> SSLDDKPQFPGASAEFIDKLEFIQPNVISGIPIYRVMDRQGQIINPSEDPHLPKEKVLKLYKSMTLLNTMDRILYESQRQGRISFYMTNYGEEGTHVGSAAALDNTDLVFGQYREAGVLMYRDYPLELFMAQCYGNISDLGKGRQMPVHYGCKERHFVTISSPLATQIPQAVGAAYAAKRANANRVVICYFGEGAASEGDAHAGFNFAATLECPIIFFCRNNGYAISTPTSEQYRGDGIAARGPGYGIMSIRVDGNDVFAVYNATKEARRRAVAENQPFLIEAMT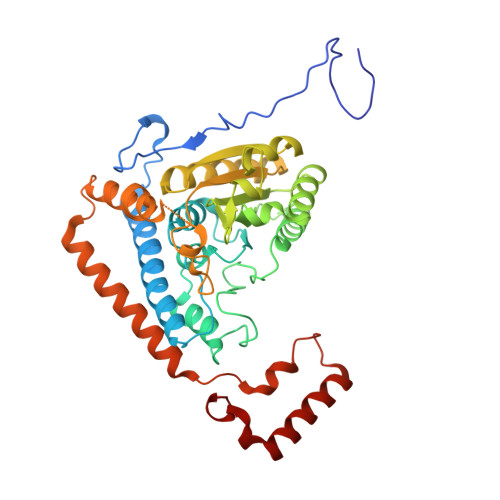YRIGHHSTSDDSSAYRSVDEVGYWDKQDHPISRLRHYLLSQGWWDEEQEKAWRKQSRRKVMEAFEQAERKPKPNPNLLFSDVYQEMPAQLRKQQESLARHLQTYGEHYPLDHFDK> MDPSKDSKAQVSAAEAGITGTWYNQLCSTFIVTAGADGALTGTYESCVGNAESRYVLTGRYDSAPATDGSGTALGWTVAWKNNYRNAHSATTWSGQYVGGAEARINTQWLLTSGTTEANAWKSTLVGHDTFTKVKPSAASIDAAKKAGVNNGNPLDAVQQ

Streptavidin is a 66-kDa, homotetrameric biotin-binding protein first isolated from the bacterium Streptomyces avidinii. The streptavidin–biotin complex has an equilibrium dissociation constant of 4 × 10–14 M, one of the strongest non-covalent interactions found in nature. The loop connecting β-strands three and four, which is often called “loop 3–4” (residues 45–52), also makes important contributions to biotin binding. When biotin is absent, this loop appears to be highly flexible and dynamically disordered, but it closes upon ligand binding, further burying biotin in the pocket.

The crystal structure of oxidized M112 in complex with biotin shows that the detailed geometry of the M112 disulfide bond differs from the prediction provided by Disulfide by Design 2.0 arising from a steric clash between the sulfur of Cys-26 and the oxygen of the backbone carbonyl group of Leu-25. The crystal structure reveals how a small but significant rotation along the Cys-26 N-Cα bond between Leu-25 and Cys-26 is able to resolve this clash. However, this change also leads to a conformational change in loop 1–2 (residues 23–27) that shifts the side chains of Leu-25 and Asn-23 away from the biotin binding site. The electron density corresponding to the side chain of Leu-25 is very weak and suggests an increase in disorder or conformational flexibility for the side chain in addition to a shift in its position away from the well-ordered contacts formed in the biotin-bound state of wild-type streptavidin. Additionally, the hydrogen bond between the nearby residue Asn-23 and the biotin ureido oxygen is lengthened to 3.7 Å compared to 3.0 Å in wild-type streptavidin; the disruption of this hydrogen bond has been predicted to be an early step in biotin dissociation from molecular dynamics simulations. Comparing the structures of wild-type streptavidin with the oxidized form of M112 suggests that the rigidity of loop 1–2 and the formation of close contacts between biotin and the loop, especially Leu-25 and Asn-23, make important contributions for binding affinity. Consistent with the structural observations of strain induced by the formation of the disulfide bond in M112 and quite unlike the formation of the disulfide bond in M88, the M112 disulfide bond forms very slowly even in the presence of 1,000-fold molar excess of oxidized glutathione, with pseudo-first order rate constants of 0.14 ± 0.02 h−1 (21 °C) and 0.41 ± 0.06 h−1 (37 °C) (half-lives of 5 and 1.6 h, respectively). The much slower rate of disulfide bond formation in M112 compared to M88 is likely related to the strain induced by disulfide bond formation and the destabilizing conformational change required for loop 1–2 to accommodate the formation of the new disulfide bond.ethyl 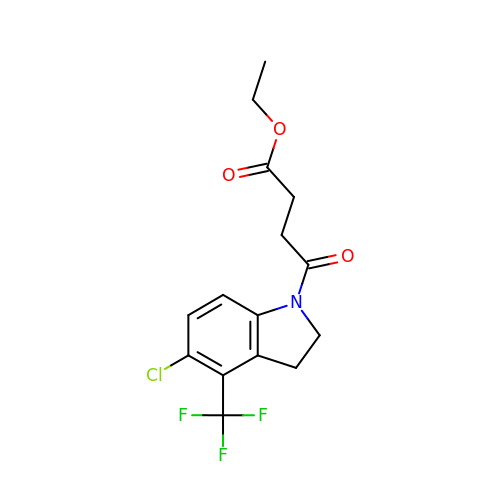4-[5-chloranyl-4-(trifluoromethyl)-2,3-dihydroindol-1-yl]-4-oxidanylidene-butanoate | C15 H15 Cl F3 N O3 | RYLCYWNNCGQOCH-UHFFFAOYSA-N>MAGSATVEKRLDFGLLGPLQMTIDGTPVPSGTPKQRAVLAMLVINRNRPVGVDALITALWEEWPPSGARASIHSYVSNLRKLLGGAGIDPRVVLAAAPPGYRLSIPDNTCDLGRFVAEKTAGVHAAAAGRFEQASRHLSAALREWRGPVLDDLRDFQFVEPFATALVEDKVLAHTAKAEAEIACGRASAVIAELEALTFEHPYREPLWTQLITAYYLSDRQSDALGAYRRVKTTLADDLGIDPGPTLRALNERILRQQPLDAKKSAKTTAAGTVTVLDQRTMASGQQAVAYLHDIASGRGYPLQAAATRIGRLHDNDIVLDSANVSRHHAVIVDTGTNYVINDLRSSNGVHVQHERIRSAVTLNDGDHIRICDHEFTFQISAGTHGGT[2x];>SLEVTEADT[2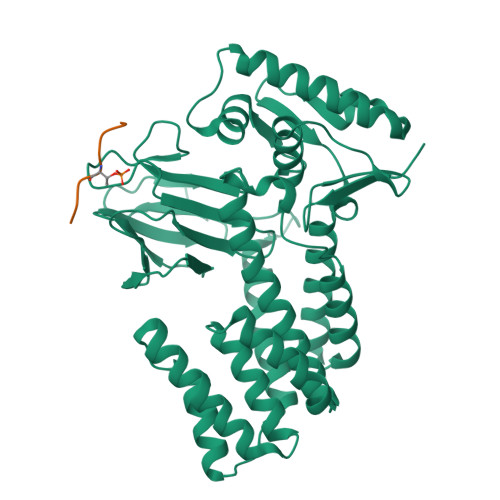x]>MEGTGVVAVYGNGAITEAKKSPFSVKVGLAQMLRGGVIMDVVNAEQARIAEEAGACAVMALERVPADIR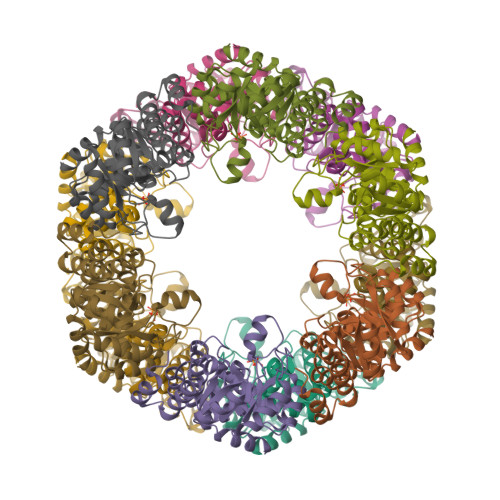AQGGVARMSDPQMIKEIKQAVTIPVMAKARIGHFVEAQILEAIGIDYIDESEVLTLADEDHHINKHNFRIPFVCGCRNLGEALRRIREGAAMIRTKGEAGTGNIIEAVRHVRSVNGDIRVLRNMDDDEVFTFAKKLAAPYDLVMQTKQLGRLPVVQFAAGGVATPADAALMMQLGCDGVFVGSGIFKSGDPARRARAIVQAVTHYSDPEMLVEVSCGLGEAM[4x]>MWKDKEFQVLFVLTILTLISGTIFYSTVEGLRPIDALYFSVVTLTTVGSDISPQTDFGKIFTILYIFIGIGLVFGFI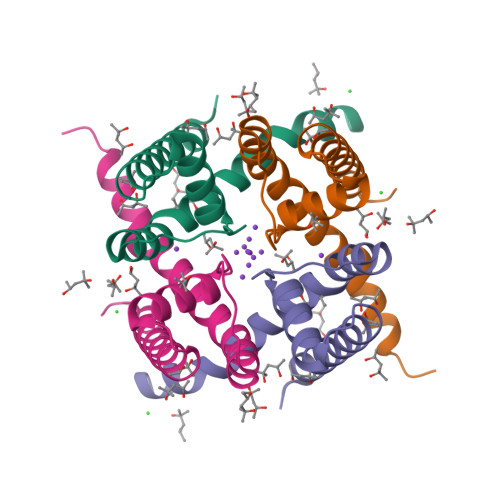HKLAVNVQLPSILSNLVPR[2x]OPEN FORM - PENICILLIN 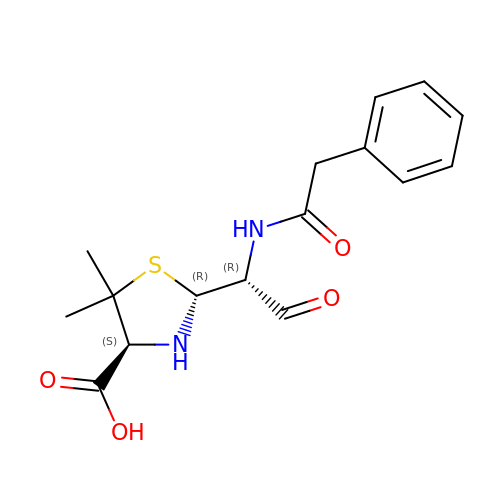G | C16 H20 N2 O4 S | OGFZUTGOGYUTKZ-KWCYVHTRSA-N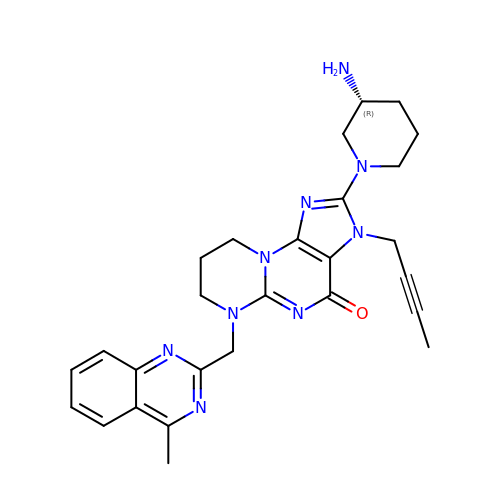2-[(3R)-3-aminopiperidin-1-yl]-3-(but-2-yn-1-yl)-6-[(4-methylquinazolin-2-yl)methyl]-6,7,8,9-tetrahydropyrimido[2,1-b]purin-4(3H)-one | C27 H31 N9 O | QWESHPQYRLOVFN-LJQANCHMSA-N> MSGSLSRGNGGKKVLNKNQLLKRNRIRNARSIRAEAVAASSTKTGTPSDLSESGSKLNVDQFISSRQFEVKQLQLAMHNSKAASSTRIFQALPRKLRRRTASHNVRRIPKRMRNRALREMRKSDQQDVLKGSSASSRKAHGLNAKQLYKARMSIKLLRLASKSTSMKLSMPPEVTSSNCHVRQKIKTLKRMIKESSTANPNIKLLNNRMGSYDCTGVNELAPIPKGRVKYTKRQKHFAWLPTHIWNAKRSHMMKRWGYQMVWAPTQKCFKLTHRLGGDTCSSDGALCMDSSYIGTIIVKDKSNDSEGDFLKSIIGKLTAERANLRKYREGQVLFQGLIYSFNEENGEDSTKPLGPCDVFWVQKDTAIIRLHPSIYTQVFNILLQHKEKLTVQDCRYSLASVTLKGAKALESLASCLRSTEYSKSFEQFKMVSMITDHNALPQRCTFAFEAIDPRHLAAPKKLNDSQRKTVNSDDILSLHENYPQDEINAVFNELCDPESRTQSYNNQNTLKEISARRYKLLTATPNSINKTTVPFKESDDPSIPLVIIRRLKTRDWIVVLPWFWLLPLWHLLNRIPRMYHIGLRQFQQIQYENKQLYFPDDYPFTQLGYIENSFYKKEASKTKWDRKPMGKRINFEKIKDIHNTKLPAYSGEIGDFFSSDWRFLQILRNGIDYLQRNDKTLELMDSKKTGQFNAQGVRDINCVNDVLEFCKDYEAKTKAMSLSIEENIPVALCKNRKCQFRTPDSISVNSSSFSLTFFPRCIIAVSCTLLERGHPKDNARIYQVPEKDLEHWLQLAKGVYRPNGRKDHDLKIPLPEVHDLIGFITSGTYHLNCGNGMGIGFIDHHAAIRQPTRYVLIRNVGTNTYRLGEWSKISV;> MDRTQTFIKDCLFTKCLEDPEKPFNENRFQDTLLLLPTDGGLTSRLQRQQRKSKLNLDNLQKVSQLESADKQLEKRDYQRINKNSKIALREYINNCKKNTKKCLKLAYENKITDKEDLLHYIEEKHPTIYESLPQYVDFVPMYKELWINYIKELLNITKNLKTFNGSLALLKLSMADYNGALLRVTKSKNKTLIGLQGIVIWDSQKFFIMIVKGNIIDEIKCIPKKGTVFQFEIPISDDDDSALRYSILGDRFKYRSVDRAGRKFKSRRCDDMLYYIQN;> MVRLKSRYILFEIIFPPTDTNVEESVSKADILLSHHRASPADVSIKSILQEIRRSLSLNLGDYGSAKCNSLLQLKYFSNKTSTGIIRCHREDCDLVIMALMLMSKIGDVDGLIVNPVKVSGTIKKIEQFAMRRNSKILNIIKCSQSSHLSDNDFIINDFKKIGRENENENEDD;> MINGVYYNEISRDLDISSSTQCLRFLKETVIPSLANNGNNSTSIQYHGISKNDNIKKSVNKLDKQINMADRSLGLQQVVCIFSYGPHIQKMLSILEIFKKGYIKNNKKIYQWNKLTSFDIKREGRNELQEERLKVPILVTLVSDSEIIDLNLHSFTKQ;> MALKKNTHNKSTKRVTKHPSLKTLTHKQIHTTIFVKSTTPYVSALKRINKFLDSVHKQGSSYVAVLGMGKAVEKTLALGCHFQDQKNKKIEVYTKTIEVLDEVITEGQADIDMESDVEDDDKETQLKKRAVSGVELRIYV;> MGKKTFREWQYFKLSITSFDQDVDDAHAIDQMTWRQWLNNALKRSYGIFGEGVEYSFLHVDDKLAYIRVNHADKDTFSSSISTYISTDELVGSPLTVSILQESSSLRLLEVTDDDRLWLKKVMEEEEQDCKCI;>[2x]MLVDLNVPWPQNSYADKVTSQAVNNLIKTLSTLHMLGYTHIAINFTVNHSEKFPNDVKLLNPIDIKRRFGELMDRTGLKLYSRITLIIDDPSKGQSLSKISQAFDIVAALPISEKGLTLSTTNLDIDLLTFQYGSRLPTFLKHKSICSCVNRGVKLEIVYGYALRDVQARRQFVSNVRSVIRSSRSRGIVIGSGAMSPLECRNILGVTSLIKNLGLPSDRCSKAMGDLASLVLLNGRLRNKSHKQTIVTGGGSGNGDDVVNDVQGIDDVQTIKVVKRSMDAEQLGHASKRHKP;> MNKDQAEKYQERSLRQKYNLLHVLPTLNSRALSGLYYKNFHNSVKRYQIMLPEQLKSGKFCSHCGCVYVPNFNASLQLTTNTEQGDSDELGGESMEGPKKCIQVNCLNCEKSKLFEWKSEFVVPTFGQDVSPMINSTSSGKVSYAVKKPQKSKTSTGKERSKKRKLNSLTNLLSKRNQEKKMEKKKSSSLSLESFMKS;> MDEMDNVIRSLEQEYRLILLLNHRNKNQHRAASWYGSFNEMKRNCGQIITLFSSRRLQAKRLKDVEWVKLHRLLQRALFRQLKRWYWQFNGVIALGQFVTLGCTLVTLLANVRALYMRLWEINETEFIRCGCLIKNLPRTKAKSVVNDVEELGEIIDEDIGNNVQENELVITSIPKPLTENCKKKKKRKKKNKSAIDGIFG

Ribonuclease (RNase) MRP, a site-specific endoribonuclease, is a ribonucleoprotein complex (RNP) comprising a catalytic RNA moiety and multiple (ten in Saccharomyces cerevisiae) protein components. Known RNase MRP functions include its participation in the maturation of rRNA and in the metabolism of specific mRNAs involved in the regulation of the cell cycle. RNase MRP appears to have split from the RNase P lineage early in the evolution of eukaryotes, acquiring distinct substrate specificity and cellular functions. S. cerevisiae RNase MRP and RNase P share eight proteins (Pop1, Pop3, Pop4, Pop5, Pop6, Pop7, Pop8, and Rpp1 (two copies)); RNase MRP protein Snm1 has a homolog in RNase P (Rpr2), while Rmp1 is found only in RNase MRP.

Here, we report a cryo-EM structure of the S. cerevisiae RNase MRP holoenzyme solved to a nominal resolution of 3.0 Å. The resultant map had an overall resolution of 3.0 Å, with the central regions as good as 2.5 Å. The final model included all known components of RNase MRP, except for a peripheral protein Pop3. The proteins are forming a clamp-like structure embedding RNA and protecting most of it from the solvent, consistent with prior biochemical data. RNase MRP RNA forms an essentially single-layered structure dominated by coaxially stacked helical regions. The fold of the C-domain of RNase MRP RNA is remarkably similar to the structurally conserved fold of the C-domains found in RNases P from all domains of life, including yeast RNase P. Pop1, the largest protein component of RNase MRP, forms the main structural brace in the RNP. At the same time, the N-terminal part of Pop1 engages mostly the S-domain RNA, which is different in RNase MRP and RNase P. The N-terminal part of Pop1 undergoes RNA-driven structural remodeling and adopts distinct conformations in the two RNPs. The structures of the S-domains of RNase MRP and RNase P differ (above), and the part of Pop4 that engages the S-domain RNA undergoes RNA-driven structural remodeling: the long alpha helix α3 found in RNase MRP Pop4 is disrupted in RNase P. In RNase MRP, the N-terminal part of α3 is involved in extensive interactions with the L5 RNA loop, stabilizing its structure, whereas in RNase P the corresponding fragment of Pop4 is rotated ~135° and engages stem P9. RNase MRP protein Rmp1 is a core RNase MRP protein involved in extensive interactions with the RNA component, binding primarily to the foundation of the P15 stem, as well as to the J7/9 region and stem P9. Interactions of Rmp1 with the foundation of the P15 stem result in a ~45° change in the stem’s orientation compared to that in RNase P. Rmp1 binds in the vicinity of the catalytic center of the enzyme and is involved in the formation of the substrate binding pocket of RNase MRP (below).> ADTRIGVTIYKYDDNFMSVVRKAIEKDGKSAPDVQLLMNDSQNDQSKQNDQIDV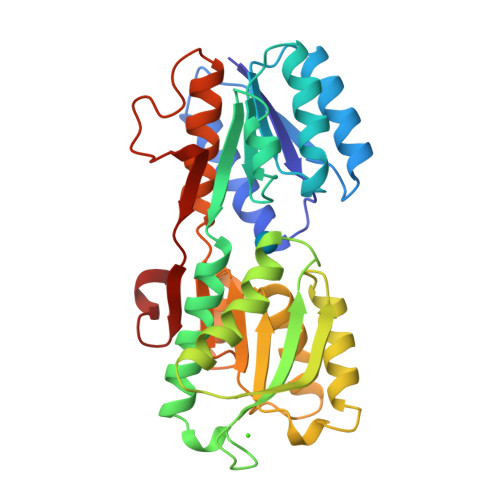LLAKGVKALAINLVDPAAAGTVIEKARGQNVPVVFFNKEPSRKALDSYDKAYYVGTDSKESGVIQGDLIAKHWQANQGWDLNKDGKIQYVLLKGEPGHPDAEARTTYVVKELNDKGIQTEQLALDTAMWDTAQAKDKMDAWLSGPNANKIEVVIANNDAMAMGAVEALKAHNKSSIPVFGVDALPEALALVKSGAMAGTVLNDANNQAKATFDLAKNLAEGKGAADGTSWKIENKIVRVPYVGVDKDNLSEFT Mitochondrial proteins CHCHD10 and CHCHD2 are mutated in rare cases of heritable FTD, ALS and PD and aggregate in tissues affected by these diseases. Here, we demonstrate that the low complexity N-terminal domains of both D10 and D2, as well as the full-length proteins, can form amyloid fibrils in vitro and in vivo. Structures of D10 and D2 fibrils assembled in vitro from the low complexity N-terminal domains of each protein show that their core comprises the most highly conserved region between the two proteins. For D10 and D2, the central conserved VAV motif forms a beta-strand that is associated with the protofilament interface in all the structures we have observed, suggesting that it may be a critical element in fibril formation and may be expected to appear in ex vivo structures as well.

Although many mutations associated with neurodegeneration are situated within the ordered cores of D10-NT and D2-NT fibrils, other disease-associated mutations occur outside these regions, including the p.R15L mutation in D10, for which we observed evidence of amyloid formation in patient fibroblasts. We solved the structure of R15L D10-NT fibrils to 3.15 Å resolution to assess whether this mutation alters fibril structure despite being outside the fibril core. The resulting structure was nearly identical to the WT D10-NT polymorph-2 structure, indicating that this mutation likely does not alter D10 fibril structure. Interestingly, however, this mutation appeared to enhance D10-NT aggregation, as assessed via ThT fluorescence, although not nearly to the extent of the S59L mutation. This mutation also leads to signal loss in NMR spectra comparable to that observed for S59L, suggesting that it too promotes intermolecular interactions. In the case of R15L and S59L D10, the introduction of a large hydrophobic residue is likely responsible for enhanced intermolecular interactions preceding aggregation. We show here that the p.R15L D10 mutation, situated far outside the D10-NT fibril core region, adopts the polymorph-2 structure of WT D10-NT, providing further evidence, albeit from a single sample and structure, that this fold is favored when the WT D10-NT sequence is preserved in the fibril core region. Although such patients are quite rare, we were able to obtain skin fibroblasts from patients with the p.R15L disease-associated D10 mutation. Staining of these cells with the amyloid-specific dye Thioflavin S (ThioS) revealed ThioS-positive punctate regions that were co-labeled by an antibody against D10, indicating that these cells contain amyloid aggregates, likely containing D10.

>MPRGSRSAASRPASLPAAPSAHPPAHPPPSAAAPAPAPSGQPGLMAQMATTAAGVAVGSAVGHVMGSALTGAFSGGSSEPSQPAVQQAPTPAAPQPLQ[18x]>[2x]GSHMASPNGQTKPLPALKLALEYIVPAMNKHGICVVDDFLGKETGQQIGDEVRALHDTGKFTDGQLVSQKSDSSKDIRGDKITWIEGKEPGCETIGLLMSSMDDLICHCNGKLGSYKINGRTKAMVACYPGNGTGYVRHVDNCNGDGRCVTCIYYLNKDWDAKVSGGILRIFPEGKAQFADIEPKFDRLLFFWSDRRNPHEVQPAYATRYAITVWYFDADETAAAKVKYLTGEKGVRVELNKPSDSVGKDVF;>[2x]DACTLLAPAAGDTIISLCF

The ferrous iron and 2-oxoglutarate (2OG)-dependent HIF prolyl hydroxylases (PHDs/EGLNs) catalyse trans-4-prolyl hydroxylations on HIFα subunits, thus promoting their binding to the von Hippel–Lindau protein (VHL), a targeting component of a ubiquitin E3 ligase, and signalling for HIFα degradation under normoxic conditions. The PHD-catalysed hydroxylations of HIF-1α/HIF-2α in higher animals occur in amino- and carboxy-terminal oxygen-dependent degradation domains (NODD and CODD). The three human PHDs exhibit different NODD/CODD selectivities, with PHD3 being substantially more selective for CODD than PHD1/2 (refs 16). Biophysical analyses employing crystallography and NMR reveal that the molecular basis of PHD isoform and variant selectivity involves enzyme–substrate interactions involving β2/β3 loop residues (that bind the LXXLAP motif) and helices α3 and α4, regions which display sequence variations between the PHD isoforms.

A PHD2 R396T variant, present in breast carcinoma, and an R396A variant efficiently hydroxylate NODD, but both manifest loss of CODD activity. We then used a ‘disulfide cross-linking' strategy to form stable PHD2.Mn.NOG.NODD complexes, where PHD2QM1 (C201A/P317C/R281C/R398A) or PHD2QM2 (C201A/V314C/R281C/R398A) and NODDDC (L397C/D412C) are cross-linked via appropriately positioned cysteines. In the PHD2.CODD structure, Arg396PHD2 (α4) is positioned to salt bridge with Asp571CODD; analysis of the ODD structures leads to the prediction that the R396T and R396A substitutions disrupt their interaction with Asp571CODD, but will not directly have an impact on NODD binding. Indeed, structures of R396T with/without NODD indicate how R396T substitution is tolerated for NODD binding. Interestingly, Asp571CODD is also important in VHL–HIFα binding, where it salt bridges with Arg107VHL3334; the high conservation of Arg396PHD2 and Arg107VHL implies that both these interactions are important in PHD–VHL evolution.> MSGNMDEAVSGNMDEAVSAGKDVRIARWVATIAGLLGFVLSVSIPLLPVTQTTATLNWPQQGRLDNVTAPLISQAPLELTATVPCSVVRDLPPEGGLVFGTAPAEGRDA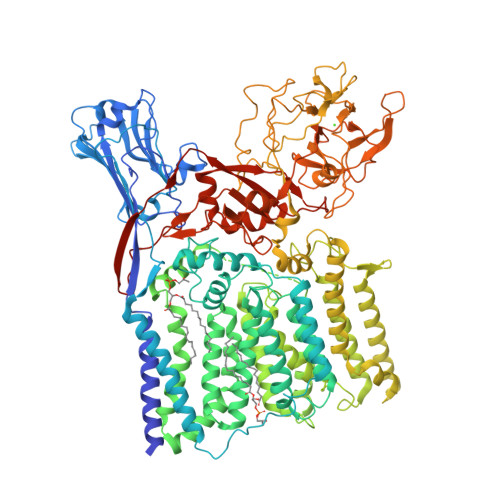ALNAMLVNVTETRVDVIVRNVVVASVNRDRVAGPDCQRIEITSNLDGTYADFVGLTQISGEDAGKLQRTGYPDPNLRPAIVGVFTDLTGPAPQGLSVSAEIDTRFTTHPTALKLAAMLLAIVSTVIALLALWRLDRLDGRRMHRLIPTRWRTVTAVDGVVVGGMAIWYVIGANSSDDGYILQMARTAEHAGYMANYFRWFGSPEDPFGWYYNVLALMTKVSDASIWIRLPDLICALICWLLLSREVLPRLGPAVAGSRAAMWAAGLVLLGAWMPFNNGLRPEGQIATGALITYVLIERAVTSGRLTPAALAITTAAFTLGIQPTGLIAVAALLAGGRPILRIVMRRRRLVGTWPLIAPLLAAGTVILAVVFADQTIATVLEATRIRTAIGPSQEWWTENLRYYYLILPTTDGAISRRVAFVFTAMCLFPSLFMMLRRKHIAGVARGPAWRLMGIIFATMFFLMFTPTKWIHHFGLFAAVGGAMAALATVLVSPTVLRSARNRMAFLSLVLFVLAFCFASTNGWWYVSNFGAPFNNSVPKVGGVQISAIFFALSAIAALWAFWLHLTRRTESRVVDRLTAAPIPVAAGFMVVVMMASMAIGVVRQYPTYSNGWANIRAFAGGCGLADDVLVEPDSNAGFLTPLPGAYGPLGPLGGEDPQGFSPDGVPDRIIAEAIRLNNPQPGTDYDWNRPIKLDEPGINGSTVPLPYGLDPKRVPVAGTYSTEAQQESRLSSAWYELPARDETERAAHPLVVITAAGTITGESVANGLTTGQTVDLEYATRGPDGTLVPAGRVTPYDVGPTPSWRNLRYPRSEIPDDAVAVRVVAEDLSLSQGDWIAVTPPRVPELQSVQEYVGSDQPVLMDWAVGLAFPCQQPMLHANGVTEVPKFRISPDYYAKLQSTDTWQDGINGGLLGITDLLLRASVMSTYLSQDWGQDWGSLRKFDTVVEATPAELDFGSQTHSGLYSPGPLRIRPAENLYFQGWSHPQFEK>[2x]GVALGATRVIYPAGQKQ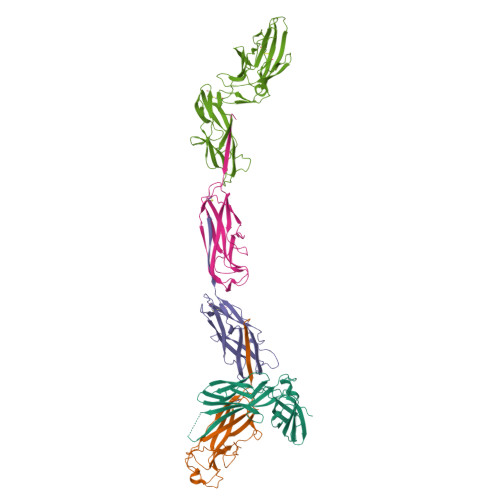EQLAVTNNDENSTYLIQSWVENADGVKDGRFIVTPPLFAMKGKKENTLRILDATNNQLPQDRESLFWMNVKAIPSMDKSKLTENTLQLAIISRIKLYYRPAKLALPPDQAAEKLRFRRSANSLTLINPTPYYLTVTELNAGTRVLENALVPPMGESTVKLPSDAGSNITYRTINDYGALTPKMTGVME;>[4x]ADSTITIRGYVRDNGCSVAAESTNFTVDLMENAAKQFNNIGATTPVVPFRILLSPCGNAVSAVKVGFTGVADSHNANLLALENTVSAAAGLGIQLLNEQQNQIPLNAPSSALSWTTLTPGKPNTLNFYARLMATQVPVTAGHINATATFTLEYQ;>ADVTITVNGKVVAKPCTVSTTNATVDLGDLYSFSLMSAGAASAWHDVALELTNCPVGTSRVTASFSGAADSTGYYKNQGTAQNIQLELQDDSGNTLNTGATKTVQVDDSSQSAHFPLQVRALTVNGGATQGTIQAVISITYTYS[2x];>[2x]FACKTANGTAIPIGGGSANVYVNLAPAVNVGQNLVVDLSTQIFCHNDYPETITDYVTLQRGSAYGGVLSSFSGTVKYNGSSYPFPTTSETPRVVYNSRTDKPWPVALYLTPVSSAGGVAIKAGSLIAVLILRQTNNYNSDDFQFVWNIYANNDVVVPTGGCDVSARDVTVTLPDYPGSVPIPLTVRCDQTQSVSYTLSGSVADAGNSIFTNTASFSPAQGVGVQLTRNGTIIPANNTVSLGAVGTSAVSLGLTANYARTGGQVTAGNVQSIIGVTFVYQ5-(4-MORPHOLIN-4-YL-PHENYLSULFANYL)-2,4-QUINAZOLINEDIAMINE 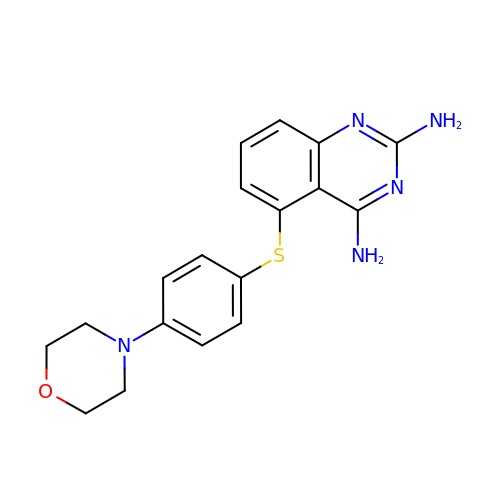| C18 H19 N5 O S | CZLWCJRHDBTCGQ-UHFFFAOYSA-N> DFRGVVDSCCRNSCSFSTLRAYC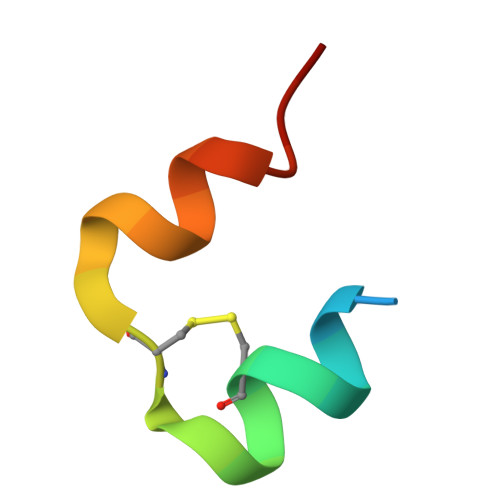DS>[2x]MEGSEPVAAHQGEEASCSSWGTGSTNKNLPIMSTASVEIDDALYSRQRYVLGDTAMQKMAKSHVFLSGMGGLGLEIAKNLVLAGIKAVTIHDTEKCQAWDLGTNFFLSEDDVVNKRNRAEAVLKHIAELNPYVHVTSSSVPFNETTDLSFLDKYQCVVLTEMKLPLQKKINDFCRSQCPPIKFISADVHGIWSRLFCDFGDEFEVLDTTGEEPKEIFISNITQANPGIVTCLENHPHKLETGQFLTFREINGMTGLNGSIQQITVISPFSFSIGDTTELEPYLHGGIAVQVKTPKTVFFESLERQLKHPKCLIVDFSNPEAPLEIHTAMLALDQFQEKYSRKPNVGCQQDSEELLKLATSISETLEEKPDVNADIVHWLSWTAQGFLSPLAAAVGGVASQEVLKAVTGKFSPLCQWLYLEAADIVESLGKPECEEFLPRGDRYDALRACIGDTLCQKLQNLNIFLVGCGAIGCEMLKNFALLGVGTSKEKGMITVTDPDLIEKSNLNRQFLFRPHHIQKPKSYTAADATLKINSQIKIDAHLNKVCPTTETIYNDEFYTKQDVIITALDNVEARRYVDSRCLANLRPLLDSGTMGTKGHTEVIVPHLTESYNSHRDPPEEEIPIATLKNFPNAIEHTLQWARDEFEGLFKQPAENVNQYLTDPKFVERTLRLAGTQPLEVLEAVQRSLVLQRPQTWADCVTWACHHWHTQYSNNIRQLLHNFPPDQLTSSGAPFWSGPKRCPHPLTFDVNNPLHLDYVMAAANLFAQTYGLTGSQDRAAVATFLQSVQVPEFTPKSGVKIHVSDQELQSANASVDDSRLEELKATLPSPDKLPGFKMYPIDFEKDDDSNFHMDFIVAASNLRAENYDIPSADRHKSKLIAGKIIPAIATTTATVSGLVALEMIKVTGGYPFEAYKNCFLNLAIPIVVFTETTEVRKTKIRNGISFTIWDRWTVHGKEDFTLLDFINAVKEKYGIEPTMVVQGVKMLYVPVMPGHAKRLKLTMHKLVKPTTEKKYVDLTVSFAPDIDGDEDLPGPPVRYYFSHDTD;> TLTVHVRSEEWDLMTFDANPYDSVKKIKEHVRSKTKVPVQDQVLLLGSKILKPRRSLSSYGIDKEKTIHLTLKVVKPSDEELPLFLVESGDEAKRHLLQVRRSSSVAQVKAMIETKTGIIPETQIVTLNGKRLEDGKMMADYGIRKGNLLFLASYSIGG

The covalent modification of target proteins with ubiquitin or ubiquitin-like modifiers is initiated by E1 activating enzymes, which typically transfer a single modifier onto cognate conjugating enzymes. UBA6 is an unusual E1 since it activates two highly distinct modifiers, ubiquitin and FAT10. In the presence of Mg-ATP, E1 catalyzes the acyl-adenylation of ubiquitin, initially forming a ubiquitin-AMP adduct. Subsequently, the E1 catalytic cysteine attacks the ubiquitin-AMP intermediate to form a thioester bond between the cysteine and the C-terminal glycine of ubiquitin, resulting in the formation of a covalent E1~ubiquitin adduct.

Since extensive initial crystallization attempts with wild-type UBA6 did not result in well diffracting crystals, a chimeric protein, referred to as UBA6chim, was utilized. In this protein the SCCH domain (residue 623 to 889) of UBA6 was replaced with its counterpart (residue 631 to 889) from human UBA1, resulting in a protein with enhanced stability. The overall structure of the UBA6chim-FAT10 C0 complex revealed that FAT10 covers the AAD, IAD and 3HB domains of UBA6chim and engages in numerous interactions distributed over a smaller and a larger interface involving the NTD and CTD, respectively. While T133 engages in limited van der Waals interactions involving its side chain Cβ and Cγ atoms, more prominent hydrophobic contacts are formed by L155, F157 and A159 of FAT10 with F316 in the IAD as well as F925, V934, and, to a more limited extent, T936, which are both located in the AAD. Second, the C-terminal tail of FAT10 is threaded underneath the crossover loop towards the ATP binding site with the C-terminal G165 being in close proximity to where the α-phosphate resides in the UBA6-ATP complex. The UBA6chim-FAT10 structure clearly revealed that the same binding pocket used by Uba1 to recognize R72 of ubiquitin is recruited for the binding of Y161 of FAT10. In contrast to the polar interactions involving the recognition of R72, Y161 is recognized predominantly by hydrophobic interactions involving H599 and H614, which are replaced by Asn and Ser (N574 and S589 in Uba1; N606 and S621 in UBA1). In contrast to the hypothesis that the NTD of FAT10 is placed in between the AAD and FCCH and interacts with these domains (see “Comparison of the UBA6 and Uba1 structures”), it is oriented in such a way that it exclusively interacts with the 3HB inserted into the IAD. These interactions are polar and primarily rely on the electrostatic complementarity of a positively charged region in the NTD involving residues K55, K58, R60 and K61 and a negatively charged patch in the 3HB formed by E320, E324, D370 and D374, with S64 of FAT10 and N318 of UBA6 contributing additional polar interactions.> MSEWWKEAVVYQIYPRSFYDANGDGFGDLQGVIQKLDYIKNLGADVIWLSPVFDSPQDDNGYDISDYKNMYEKFGTNEDMFQLIDEVHKRGMKIVMDLVVNHTSDEHAWFAESRKSKDNPYRDYYLWKDPKPDGSEPNNWGSIFSGSAWTYDEGTGQYYLHYFSKKQPDLNWENEAVRREVYDVMRFWMDRGVDGWRMDAIGSISKYTDFPDYETDHSRSYIVGRYHSNGPRLHEFIQEMNREVLSHYDCMTVGEANGSDIEEAKKYTDASRQELNMIFTFE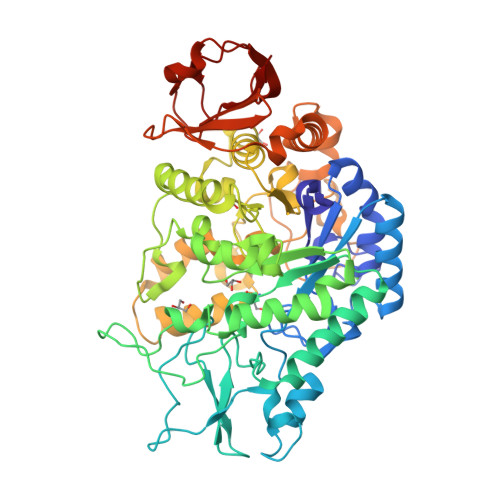HMDIDKEQNSPNGKWQIKPFDLIALKKTMTRWQTGLMNVGWNTLYFENHDQPRVISRWGNDRKLRKECAKAFATVLHGMKGTPFIYQGEEIGMVNSDMPLEMYDDLEIKNAYRELVVENKTMSEKEFVKAVMIKGRDHARTPMQWDAGKHAGFTAGDPWIPVNSRYQDINVKESLEDQDSIFFYYQKLIQLRKQYKIMIYGDYQLLQENDPQVFSYLREYRGEKLLVVVNLSEEKALFEAPPELIHERWKVLISNYPERADLKSISLKPYEAVMGISI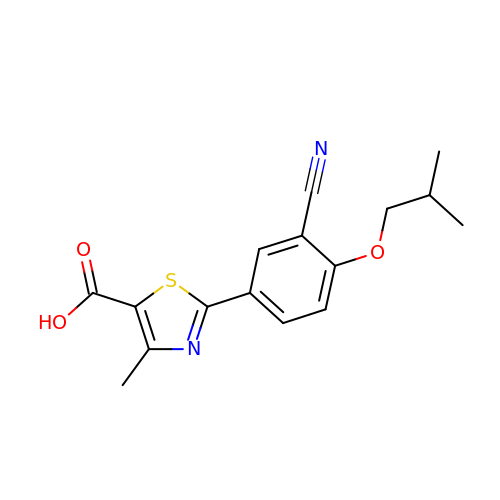2-(3-CYANO-4-ISOBUTOXY-PHENYL)-4-METHYL-5-THIAZOLE-CARBOXYLIC ACID | C16 H16 N2 O3 S | BQSJTQLCZDPROO-UHFFFAOYSA-N>[2x]GPVGEPVASEINEASKVSSRLLTQDILFRKDRQATISLPIKLPVEDIITQTCDKITYGPLKFLDLLEK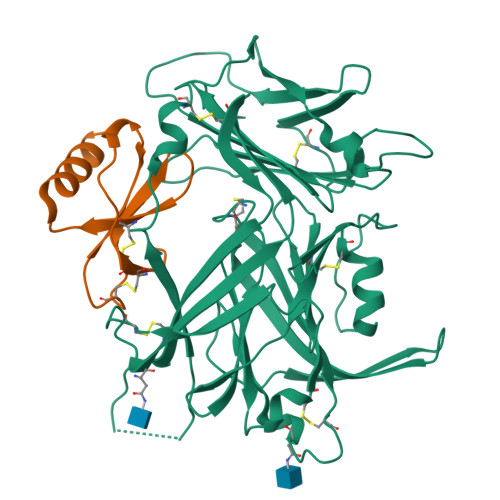ETAVLPLSTDITCPACLGRAVLVGKWECPAHVAVNESDLTVFGPNKEEHVPQFVTVQQPSDGKMQRLFFAKFLGTEESLAVLRVPGPDGHLCIQEALIHFKELSGAGVCSLWKANDSREEGLEMKQVDCLETTVLENQTCIATTLSKKIYHRLYCGERLMTGGQVSTRVLLTALGFYKRQPYTFHRVPKGMVYVHLIDSGSEDYMEYSECEEVTPGRYEDKQISYTFYTDLFQTADGEPVLASVWGTSGLKDSAYESCAFVIPTDGEEDLVPRRIMSKCYPFRLTYHPSTMTVRLDVRVEKHHGATDQGFVFLKMESGTYSEGREYYLDRVLWGEDSSTNNVLQHHHHHHHH;>[2x]MAPYGADTPTACCFSYSRKIPRQFIVAYFETSSLCSQPGVIFLTKRNRQICADSKETWVQEYITDLELNA The housekeeping enzyme glucose 6-phosphate dehydrogenase (G6PD) (EC 1.1.1.49) is the first and rate-limiting enzyme of the PPP. It catalyzes the oxidation of glucose 6-phosphate (G6P) originating from glycolysis to 6-phospho-D-glucono-1,5-lactone (6PL), whereby the cofactor NADP+ is reduced to NADPH. In the present study, we describe the crystal structures of Leishmania donovani G6PD (LdG6PD), both native and complexed with one or both substrates. The LdG6PD monomer contains three domains: an N-domain (Q5-K49), the NADP+ binding “Rossmann-like” domain (residues D50-I248), and a β + α domain (residues D249-K552).

To investigate a potential function of the helical N-domain conserved in Kinetoplastida G6PDs, we generated a truncation mutant lacking the N-domain that includes residues 1–59 (LdG6PD60-562). Crystals containing only NADP(H) diffracted to a resolution up to 1.7 Å, and crystals containing G6P or G6P and NADP(H) to 3.3 Å and 2.5 Å, respectively. The crystal of the truncated mutant LdG6PD60–562 obeyed C222 symmetry with one monomer in the AU and diffracted to 1.9 Å. In contrast to the wt and LdG6PDC138S crystals, which contain the physiological dimer in the AU, the truncation mutant LdG6PD60–562 crystallized in an orthorhombic space group (C222) with one molecule in the AU. Consequently, the physiological dimer is formed by a crystallographic two-fold rotation axis. However, our usual tetramer cannot be constructed via crystallographic symmetry operations. Instead, a different tetramer is formed via C222 symmetry operations, which interestingly resembles the G6PD tetramer of related Trypanosoma species. Here, the LdG6PD dimer–dimer interface is mainly formed by salt bridges (R268, K324, R326, D335, E336, and D393), keeping the dimers in a back-to-back orientation. In accordance with these structural results and in contrast to the stable dimer-to-tetramer equilibrium of LdG6PD wt, the tetramer was no longer visible in the SEC profiles of LdG6PD60–562 but only a single peak corresponding to the dimer form of the mutant. However, the crystallographic and SEC observations were not reflected by impaired catalytic efficiency of the enzyme. Only minor conformational changes of the core domains in the crystal structure of LdG6PD60–562 confirmed this when compared to the wt.

> NCKVKDEQKSRALTIIVFGASGDLAKKKTFPALFDLYCGGLLPPEVNIIGYARTKVDDVEKWKHETLMKYFSNLSERGCHAEDFLKHISYFCGAYDSVDDFKRLDAVIREKENAFKGPEKGGNRLFYLALPPSVFASVCESIHKGAMPQEVGGWVRVIIEKPFGRDTKSSAELSQALEPFFDESQLYRIDHYLGKEMVQNIITTRFANRIFSAVWNASNIACVQITFKETIGTEGRGGYFDNIGIIRDVMQNHLTQILALLAMEKPRSLDAECIRDEKVSVLKCIEPITKENCVLGQYTASADGSIPGYLEDVTVPEGSTCPTFAVMRLNINNDRWAGVPFILKAGKAVEQKYVAIRIQFRDEVHPYGEATQRNELVIRAQPSEAMYVKITTKVPGLSGDLRQTHQTELDLTYHTRYDVRLPDAYESLINDALLGNSTNFVRKDELDVAWRIFTPLLHQIDSGEIKPIPYQAGTRGPKEADEFIANNGFKHQKGYHWLPSNKL> LPRVKHTLVPPPFAHAHEQVAASGPVINEFEMRIIEKEVQLDEDAYLQAMTFDGSIPGPLMIVHEGDYVELTLINPPENTMPHNIDFHAATGALGGGGLTLINPGEKVVLRFKATRAGAFVYHCAPGGPMIPWHVVSGMAGCIMVLPRDGLKDHEGKPVRYDTVYYIGESDHYIPKDEDGTYMRFSDPSEGYEDMVAVMDTLIPSHIVFNGAVGALTGEGALKAKVGDNVLFVHSQPNRDSRPHLIGGHGDLVWETGKFHNAPERDLETWFIRGGSAGAA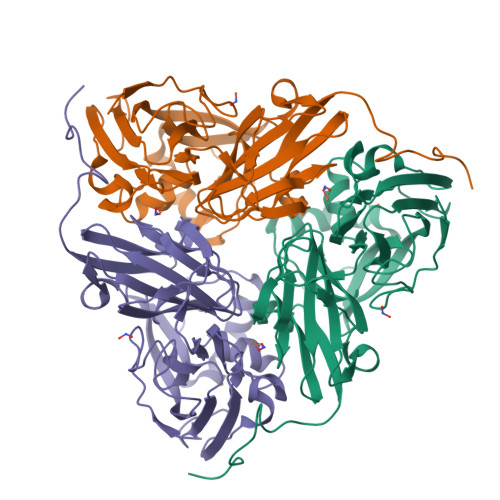LYKFLQPGVYAYVNHNLIEAVHKGATAHVLVEGEWDNDLMEQVVAPVGL>MRLELPVIPLRNTVILPHTTTPVDVGRAKSKRAVEEAMGADRLIFLVAQRDPEVDDPAPDDLYTWGVQAVVKQAMRLPDGTLQVMVEARARAQVTDYIPGPYLRARGEVFSEIFPIDEAVVRVLVEELKEAFEKYVANHKSLRLDRYQLEAVKGTSDPAMLADTIAYHATWTVAEKQEILELTDLEARLKKVLGLLSRDLERFELDKRVAQRVKEQMDTNQREYYLREQMKAIQKELGGEDGLSDLEALRKKIEEVGMPEAVKTKALKELDRLERMQQGSPEATVARTYLDWLTEVPWSKADPEVLDINHTRQVLDEDHYGLKDVKERILEYLAVRQLTQGLDVRNKAPILVLVGPPGVGKTSLGRSIARSMNRKFHRISLGGVRDEAEIRGHRRTYIGAMPGKLIHAMKQVGVINPVILLDEIDKMSSDWRGDPASAMLEVLDPEQNNTFTDHYLDVPYDLSKVFFITTANTLQTIPRPLLDRMEVIEIPGYTNMEKQAIARQYLWPKQVRESGMEGRIEVTDAAILRVISEYTREAGVRGLERELGKIARKGAKFWLEGAWEGLRTIDASDIPTYLGIPRYRPDKAETEPQVGTAQGLAWTPVGGTLLTIEVAAVPGSGKLSLTGQLGEVMKESAQAALTYLRAHTQDYGLPEDFYNKVDLHVHVPDGATPKDGPSAGITMATAIASALSRRPARMDIAMTGEVSLRGKVMPIGGVKEKLLAAHQAGIHKIVLPKDNEAQLEELPKEVLEGLEIKLVEDVGEVLEYLLLPEPTMPPVVQPSDNRQQPGAGA[5x]

The Lon protease is a AAA+ protein found in prokaryotes, archaea, and eukaryotic organelles. Lon is involved in cellular protein homeostasis by degrading damaged or misfolded abnormal proteins, which prevents these unwanted protein species from forming toxic aggregates. Lon is known to form a homohexamer; each protomer is composed of multiple domains, including an N-terminal substrate-binding globular domain (NGD), a long-helix domain (LH), a three-helix bundle (3H), a AAA+ ATPase module, and a protease domain. We show here, using cryo-electron microscopy (cryo-EM), that the activation process of the Lon AAA+ protease may involve a pentameric assembly and a substrate-dependent incorporation of the sixth protomer to form the substrate-pore-loop contacts seen in the translocating state.

To provide a comparative context, we also examined wild-type MtaLon in two states: without any nucleotide (MtaLon-Apo) and incubated with 5 mM ADP (MtaLon:ADP). Unexpectedly, both MtaLon-Y224S:ATPγS and wild-type MtaLon, whether with ADP or lacking nucleotide, predominantly formed left-handed spiral pentamers or spiral hexamers, rather than closed-ring hexamers. Surprisingly, the pentameric form consistently emerged as the most prevalent class. The pentameric assembly forms a left-handed open-spiral structure. The open-spiral pentamer forms a large gap between the protomers Ob1 and Ob5. The pentamer forms a tensegrity helix triangle (THT), consisting of three overlapping LHs from Ob1, Ob3, and Ob5, forming an interlocked, letter A-shaped structure that tethers together five protomers.> GSPEFTSQLVIMSELIELKQDGDLESLLEQHK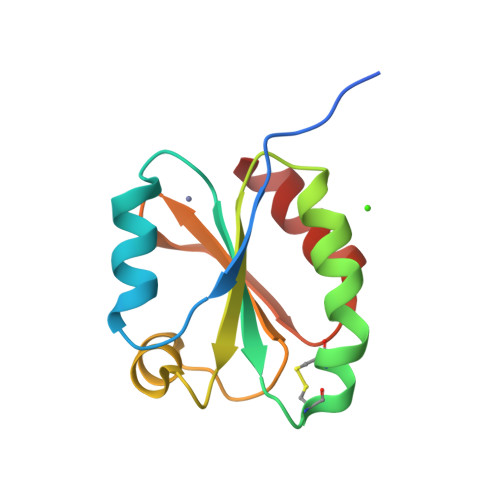NKLVVVDFFATWCGPCKTIAPLFKELSEKYDAIFVKVDVDKLEETARKYNISAMPTFIAIKNGEKVGDVVGASIAKVEDMIKKFI>[4x]SYEDQNSLLKMICQQV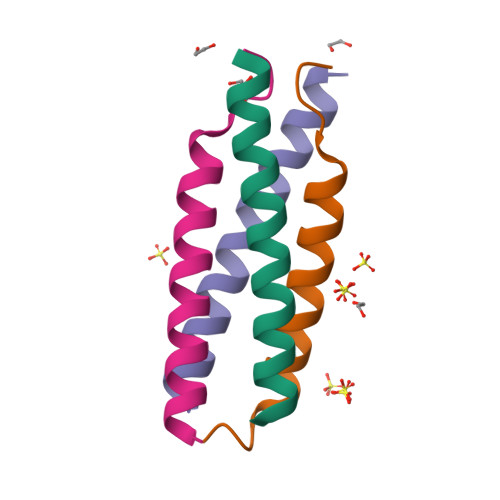EAIKKEMQELKLNS Here, we characterize the O-methyltransferases BelI and CysG, which catalyze the initial step of β-lactone formation. Employing techniques such as crystallography, computational analysis, mutagenesis, and activity assays, we identified a His-His-Asp (HHD) motif in the active sites of the two enzymes, which is crucial for binding a catalytically active calcium ion. As expected, BelI as well as CysGΔN16 adopt the class I methyltransferase Rossmann fold, characterized by a core domain of a seven-stranded β-sheet flanked by α-helices. The HHD-motif enables regiospecific C1-carboxy group methylation of their respective malic substrates.

Due to the high crystallization tendency of CysGΔN16, subsequent mutagenesis experiments were focused on this variant. Therefore, we conducted structure-based mutagenesis by introducing non-conservative alanine residues in the HHD motif to further explore the metal-binding site. In contrast, the CysGfl-H122A variant remained active across diverse metal ions but was inactivated by EDTA. Therefore, His122 is involved in metal stabilization without affecting the interaction between protein and substrate.

>[4x]GSTYDALRRQLIPSFDLLYGSAVSVVAMSVPATARILDLGAGTGLLGAALRERLPDAELLLQDRSQAMLEQARQRFADDDQVAIRVADHLDELPAGPFDAVVSALSIAHLEHQDKQDLFTRIRKILRPGGIFVNVEQVLAPTSELEKMYDRQHEAHVLASDTPAEEWAAGRERMKHDIPIDVETQIQWLRDAGFTTADCLAKDWRFATYAGWNGSC2-azanyl-9-[(2R,3R,4S,5R)-5-(hydroxymethyl)-3,4-bis(oxidanyl)oxolan-2-yl]-1-methyl-purin-6-one 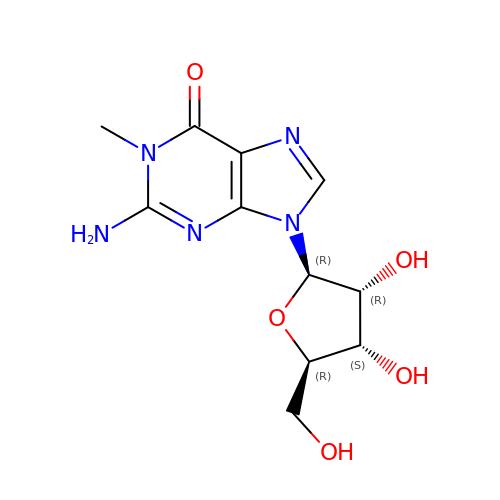| C11 H15 N5 O5 | UTAIYTHAJQNQDW-KQYNXXCUSA-N>[2x]MAHHHHHHSSGQFREFSIETIRNATSGFAAENIVSEHGERAPNVVYKGKLENQRRIAVKRFNRKSWPDSRQFLEEAKAVGQLRNHRMANLLGCCYEDEERLLIAEFMPNETLAKHLFHWESQPMKWAMRLRVALHIAQALEYCTSKGRALYHDLNAYRVLFDDDANP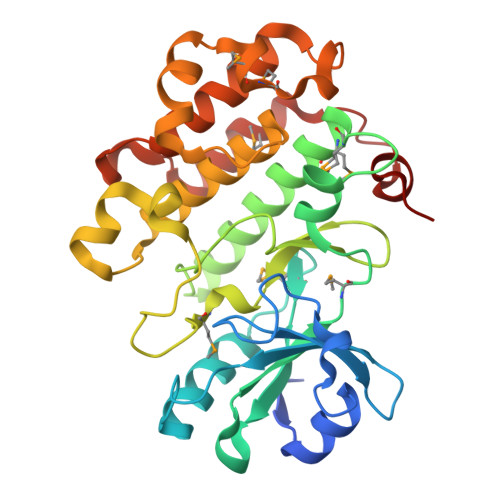RLSCFGLMKNSRDGKSYSTNLAFTPPEYLRTGRVTPESVIYSFGTLLLDLLSGKHIPPSHALDLIRDRNIQMLMDSGLEGQFSSDDGTELIRLASRCLQYEPRERPNPKSLVSAMIPLQKDLEIASHQLLGVP N'-{(1S,2S)-1-(3,5-difluorobenzyl)-2-hydroxy-2-[(2R)-4-(phenylsulfonyl)piperazin-2-yl]ethyl}-5-methyl-N,N-dipropylbenzene-1,3-dicarboxamide | C34 H42 F2 N4 O5 S | 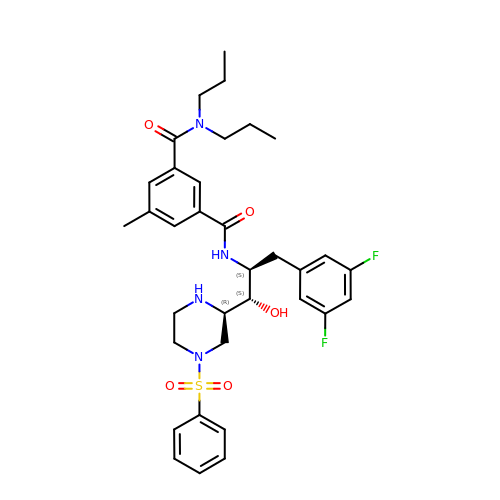KDRUCCZCGHVXGH-QAXCHELISA-N>MRSYHVVTNDTLPSALDAIAQAPRVALDTETYGSNPFNLYLPDFRLVGVAIATSPTEAWYFPVDHQDFLLRYQPANLPREAVRQAVLEALKRPVVYHNAAYDRRVLAVTLDIPLDQTYGDDTMVALHLVDENHPLGLKEWAKTLLGLEEVNADIEPPELTDEDQVEAVSKNGRRYKKKVHKLKPDWLQRLKD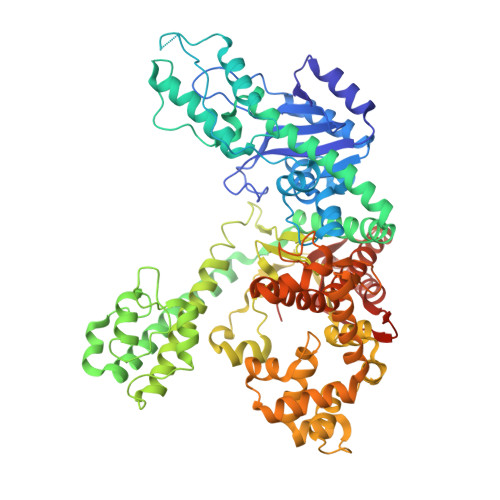AFLAVHNGGVSYSALYKLLNRAFQQLKNRGVVSYTGSFPNDFRLFPVDIAAIYALDDAMNTLALWEHVEVFFELHPKLHALYREIELPVNDVMTRATHRGVLVDKEELRRIKETIQARIEEKAQEAQELLKALIGSKASEFTNPLNSPQQLSTILYDLLGYPVVETTPNGAPSTSKTAIAKLLTLSPKDKRKAPLAKAFLEAKQAHEGLKKLLSTYTDSILEEVDPQGRLHTNFNTVGTVSGRMSSSNPNLQNLPRLLPEEVAEKPYLQGIDIRKAFVADPGYTFVSADYASMELVVCAAVSGDPTMRDLLNQGRDLHAYTARYAFKVGLDLDDKAFKEQYKDYRQKAKVVNFALIYGGTEFTLIKNFGFSEEEAKQLIQGYFEAYPVVKTWMEEVYRELEEKGFVEYPIYGYIKRMDLPQALRKLPKDKWPLVLNNDPDARKQYYASLRSCQNALIQGFSAFVVKDAIVQMQRAFEAEGLDAQVIIQVHDEIVVLAKEEHAERVAQIMVEKMEREVNGVLLKAEPEFKRTLSKVGLEHHHHHH[2x]> AAAAAAAAAAAAAAAAAAAAAAAAAAAAAAAAAAAA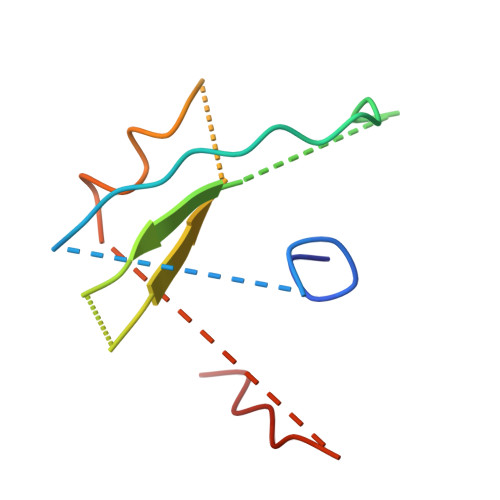AAAAAAAAAAAA> MAPVIPSNTDYPGPHHFEVTFQQSSTAKSATWTYSPLLKKLYCQIAKTCPIQIKVSTPPPPGTAIRAMPVYKKAEHVTDVVKRCPNHELGRDFNEGQSAPASHLIRVEGNNLSQYVDDPVTGRQSVVVPYEPPQVGTEFTTILYNFMCNSSCVGGMNRRPILIIITLEMRDGQVLGRRSFEGRICACPGRDRKADEDHYREAENLYFQ

The p53 family of transcription factors comprises p53 and the paralogs p63 and p73.1 Under conditions of cellular stress, all three proteins are activated to induce genes necessary for cell cycle arrest or apoptosis. All three proteins share a similar domain organization containing an N-terminal transactivation domain, a DNA-binding domain (DBD) and a C-terminal oligomerization domain (OD).9 p63 and p73 contain an additional sterile α-motif domain and an inhibitory domain at the C-terminus. Both p63 and p73 share approximately 60% sequence identity with p53 in the DBD, and DNA contact residues are strictly conserved across all three proteins. To address the potential for similar p73 assembly, we solved the high‐resolution crystal structure of the DBD of p73 as well as its complex with the ankyrin repeat and SH3 domains of ASPP2.

Crystals were obtained in space group P4332 with one protein molecule in the asymmetric unit. The final p73 structure was solved using molecular replacement and refined at a resolution of 1.8 Å (see Table 1 for data collection and refinement statistics). The entire chain was traced with the exception of the three L3 loop residues from G265 to N267, which were not visible in the electron density. The p73 structure shows a conserved domain architecture, comprising a β-sandwich scaffold consisting of two antiparallel β-sheets.27 The DNA-binding surface is constructed similarly from the large L2 and L3 loops, the S10 β-strand and a loop–sheet–helix motif that includes the L1 loop, the S2 and S2′ β-strands and the C-terminal H2 α-helix. A conserved zinc ion coordinates the L2 and L3 loops (p73 C194, H197, C258 and C262) and contributes to the stability of the overall fold. The p73 structure also includes a second metal ion trapped at the interface of a crystallographic dimer formed by the H2 helix and the C-terminal His-tag. Unusually, a disulfide bond is observed in the p73 structure between C153 (S2′) and C159 (S3), although the main‐chain atoms remain similarly placed to p53 C135 and C141, suggesting that the oxidation has limited structural significance and is most likely the result of insufficiently reducing conditions during purification. As a result, p73 residues R201–A209 adopt a markedly different conformation to p53 C182–A189. Instead, the p73 insertion induces a loose helical turn that places N204 in the equivalent position to hydrogen bond with both p73 R193 and R216. The p73 DBD is the last globular domain in the p53 family to be structurally determined. Its structure reveals a conserved fold for DNA binding but a divergent L2 loop.> KSAKDALLLWCQMKTAGYPNVNIHNFTTSWRDGMAFNALIHKHRPDLIDFDKL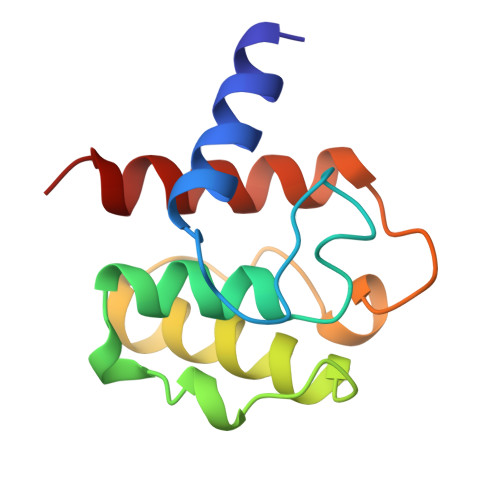KKSNAHYNLQNAFNLAEQHLGLTKLLDPEDISVDHPDEKSIITYVVTYYHYFSKM>[2x]STETLSFTPDNINADISLGTLSGKTKERVYLAEEGGRKVSQLDWKFNNAAIIKGAINWDLMPQISIGAAGWTTLGSRGGNMVDQDWMDSSNPGTWTDEARHPDTQ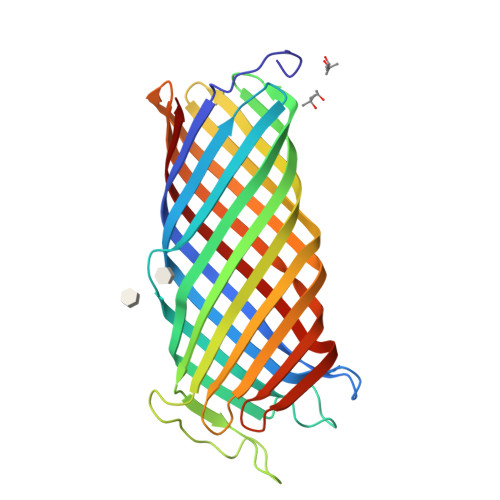LNYANEFDLNIKGWLLNEPNYRLGLMAGYQESRYSFTARGGSYIYSSEEGFRDDIGSFPNGERAIGYKQRFKMPYIGLTGSYRYEDFELGGTFKYSGWVESSDNDEHYDPKGRITYRSKVKDQNYYSVAVNAGYYVTPNAKVYVEGAWNRVTNKKGNTSLYDHNNNTSDYSKNGAGIENYNFITTAGLKYTF>MSHPHPELGRPPALPKGGLRVTPLGGLGEIGRNMTVFEYGGRLLIVDCGVLFPEEEQPGIDLILPDFTSIRDRLDDIEGIVLTHGHEDHIGGVPFLLREKPDIPLIGSKLTLALIEAKLQEHRIRPYTLEVAEGHRERVGPFDCEFVAVNHSIPDALAVAIRTPAGMVVHTGDFKMDQLPLDGRLTDLHAFARLSEEGIDLLLADSTNAEVPGFVPPERDISNVLRQVFANARKRIIVASFASHVHRIQQILDAAHEYGRRVAFVGRSMVRNMGIARDLGYLKVPPGLVVDVKTLDDLPDSEVVLVCTGSQGEPMAALSRMANRDHQIRIVNGDTVILASSLIPGNENAVYRVINGLTRWGANVVHKGNAKVHVSGHASAGELLYFYNICRPKNLMPVHGEWRH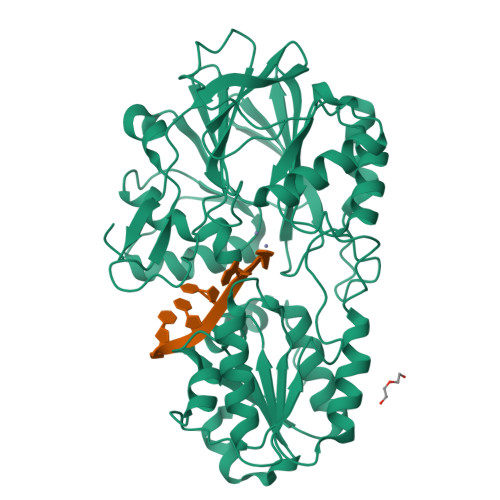LRANAELGALTGVPHDRIVIAEDGVVVDLVEGKAKITGKVQAGYVYVDGLSVGDVGEPALKDRKILGDEGIISVFVVMDSSTGKITGGPHVQARGSGIEDSAFAAVLPKVTEALERSAQDGVVEPHQMQQLIRRTLGKWVSDTYRRRPMILPVVVEV[2x]>[2x]MRVNNGLTPQELEAYGISDVHDIVYNPSYDLLYQEELDPSLTGYERGVLTNLGAVAVDTGIFTGRSPKDKYIVRDDTTRDTFWWADKGKGKNDNKPLSPETWQHLKGLVTRQLSGKRLFVVDAFCGANPDTRLSVRFITEVAWQAHFVKNMFIRPSDEELAGFKPDFIVMNGAKCTNPQWKEQGLNSENFVAFNLTERMQLIGGTWFGGEMKKGMFSMMNYLLPLKGIASMHCSANVGEKGDVAVFFGLSGTGKTTLSTDPKRRLIGDDEHGWDDDGVFNFEGGCYAKTIKLSKEAEPEIYNAIRRDALLENVTVREDGTIDFDDGSKTENTRVSYPIYHIDNIVKPVSKAGHATKVIFLTADAFGVLPPVSRLTADQTQYHFLSGFTAKLAGTERGIT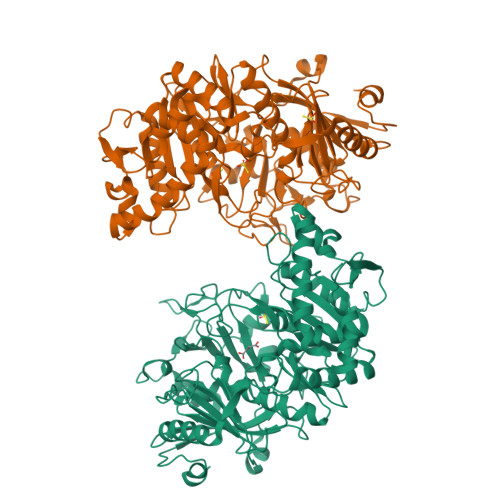EPTPTFSACFGAAFLSLHPTQYAEVLVKRMQAAGAQAYLVNTGWNGTGKRISIKDTRAIIDAILNGSLDNAETFTLPMFNLAIPTELPGVDTKILDPRNTYASPEQWQEKAETLAKLFIDNFDKYTDTPAGAALVAAGPKLHHHHHH Because intestinal β-glucuronidase (GUS) enzymes have been shown to convert a wide range of glucuronidated metabolites to their corresponding aglycones, we hypothesize that gut microbial GUS orthologs would catalyze the conversion of TSC-G to TCS. The human and mouse gut microbiome have been shown to contain hundreds of unique gut microbial GUS enzymes, which exhibit distinct substrate specificities toward varying glucuronides. Previous studies have shown that microbial GUS enzymes can be categorized into seven distinct clades based on active site architecture and/or cofactor binding. Our central finding is that specific gut microbial enzymes, notably, gut microbial GUS proteins of the Loop 1 and FMN-binding clades, mediate the colonic reactivation of TCS from its inactive glucuronide metabolite, and in doing so they drive the gut toxicity of TCS.

We focused on F. prausnitzii 2-L1 (Fp2-L1) GUS, which was the most active Loop 1 GUS protein identified from our in vitro enzymatic assays. The crystal structure of Fp2-L1 GUS was determined and refined to 2.2 Å resolution and reveals a protein tetramer with a GUS inhibitor UNC10201652 (GUSi) covalently linked to glucuronic acid in each active site. Fp2-L1 GUS was crystallized in the presence of GUSi and the reporter substrate p-nitrophenyl-glucuronide. GUSi has been shown to intercept the GUS catalytic cycle and produce the covalent GUSi-glucuronic acid adduct observed here and described previously. Using the Schrödinger molecular modeling suite, we docked TCS-G into the active site of Fp2-L1 GUS and found that Y479 and three methionines (M454, 455, and 362) are positioned to potentially contact TCS-G. Mutation of Y479 or M362 to alanine significantly reduced TCS-G processing, while mutation of M454 or M455 to alanine significantly increased TCS-G processing, perhaps by reducing steric occlusion during TCS-G turnover. We confirmed by circular dichroism that the mutant proteins did not exhibit significant structural changes compared to the wild-type enzyme, indicating that the mutations are directly responsible for the observed loss of activity with TCS-G. Furthermore, methionines 362 and 455 are unique to Fp2-L1 GUS compared to another Loop 1 GUS enzyme, E. coli GUS, that we show poorly utilizes TCS-G as a substrate (see the alignment of Fp2-L1 GUS and E. coli GUS in Supplementary Fig. S8). First, we tested the effect of GUSi on TCS-G processing in vitro and found that it inhibited the conversion of TCS-G to TCS by purified Fp2-L1 GUS enzyme, as well as several other Loop 1 GUS enzymes, in a dose-dependent manner, with IC50 values of 0.64–4.9 µM. Thus, taken together, the in vitro activity and coupled proteomic data support the conclusion that Loop 1 gut microbial GUS enzymes appear to be important drivers of TCS-G processing.

>MNNKSLLYPVVSTSRRVVSLDGMWRFSFDAKSEGVEANWANGLPESISMPVPASFCDFFTDKESREYCGDFWYETDFFVPGEWSGKDIAIRFGSATHHARIFVNGVEVAQHEGGFLPFDAVVTDIVRYNQFNKLSVLLNNELNEHMLPAGNTAVLSNGKKVAAPYFDFYNYAGIHRPVKLMALPTERILDYSVKHRLTAEGAEVDYTVTTNGDHEVTVELYDGTTKVAEATGKEGTLVVKDAKLWNVHAAYLYNIVIRIHDGSAVVDEYTEKVGIRTFEIKDGHFLLNGKPVYLRGFGKHEDADIRGRGLDLATVKRDYELMKWIGANCFRTSHYPYAEELYQMADEEGFLIIDEVPAVGFMESTMNFLAANQGNGKKVGWFEKETTPQLLANHKDALTDMIGRDKNHASVIAWSILNEPQCTSEGTEAYFKTLFDLAHELDPQKRPRTYAVVMMSLPNNSKGQQFADFISLNRYYGWYVMGGMGIVDAEAAFRKEMNGWAQVLNGRPMIFTEYGADTMPTEHKLPSVMWSQEYQNEYLDMNHNVFDSYNFVQGELVWNFADFQTTEGILRVNGNKKGIFTRQRQPKDAAFLFRARWTSLPLDYKGNQ[4x]(3R)-3-aminopyrrolidin-2-one 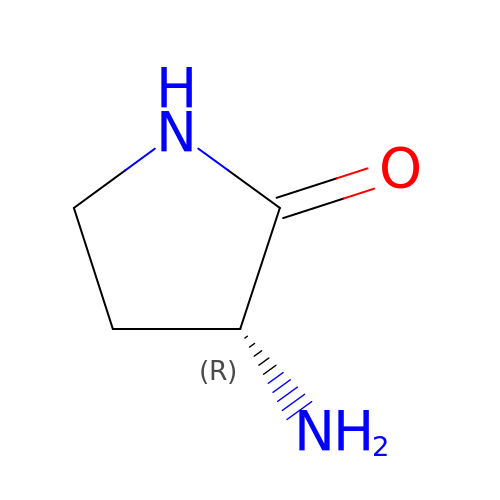| C4 H8 N2 O | YNDAMDVOGKACTP-GSVOUGTGSA-N>DPAGLLDLRQGMFAQLVAQNVLLIDGPLSWYSDPGLAGVSLTGGLSYKEDTKELVVAKAGVYYVFFQLELRRVVAGEGSGSVSLALHLQPLRSAAGAAALALTVDLPPASSEARNSAFGFQGRLLHLSAGQRLGVHLHTEARARHAWQL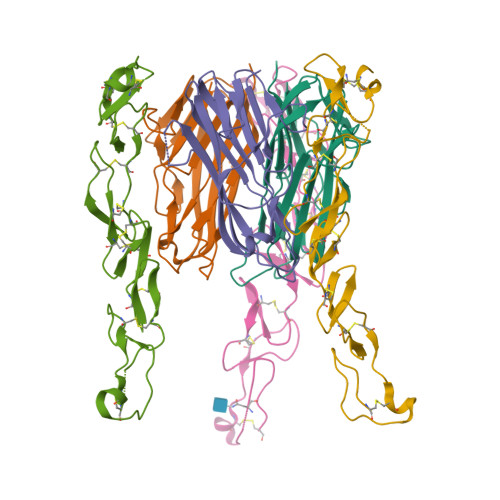TQGATVLGLFRVTPEI[6x];>[6x]SLQDPCSNCPAGTFCDNNRNQICSPCPPNSFSSAGGQRTCDICRQCKGVFRTRKECSSTSNAECDCTPGFHCLGAGCSMCEQDCKQGQELTKKGCKDCSFGTFNDQKRGICRPWTNCSLDGKSVLVNGTKERDVVCGP>[2x]MADEIAKAQVARPGGDTIFGKIIRKEIPAKIIFEDDRCLAFHDISPQAPTHFLVIPKKHISQISVAEDDDESLLGHLMIVGKKCAADLGLNKGYRMVVNEGSDGGQSVYHVHL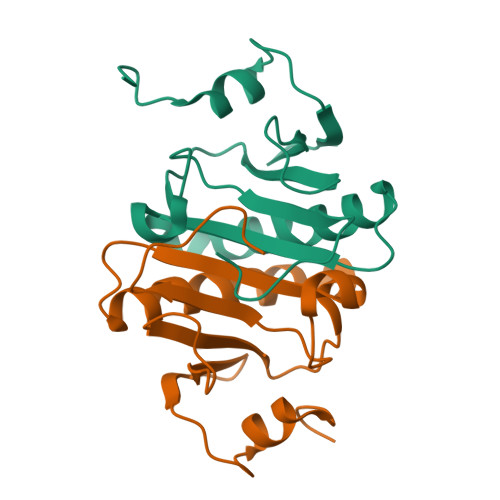AVLGGRQMHWPPG>GSHMASTPDKFNDGNLNIAYAKPTTQSSVDYNGDPNRAVDGNRNGNFNSGSVTHTRADNPSWWEVDLKKMDKVGLVKIYNRTDAETQRLSNFDVILYDNNRNEVAKKHV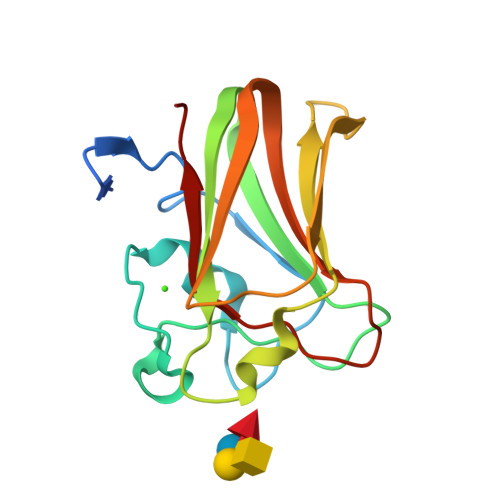NNLSGESVSLDFKEKGARYIKVKLLTSGVPLSLAEVEVFRES[2x]We use bacteriophage φ6, a member of the Cystoviridae family, as a model system to study the assembly of a complicated multi-shelled virus. The inner T=1 shell, composed of protein P1, forms a dodecahedral polymerase complex (PC) harbouring the three viral dsRNA segments (S, M, and L), the viral polymerase P2, the hexameric packaging protein P4, and the assembly cofactor P7. The expanded PC is covered by a layer of P8, forming the outer T=13 shell. Here we present the structure of φ6 NC to near-atomic resolution using electron cryomicroscopy and single particle analysis.

The six-fold symmetry of the P4 hexamer and five-fold symmetry of the icosahedral vertex beneath creates a symmetry mismatch, so that the structure of P4 cannot be resolved using conventional icosahedral reconstruction. To address this we applied the localized reconstruction method17 to P4 hexamers. Local areas corresponding to P4 hexamers were extracted from the NC images and reconstructed as single particles with six-fold symmetry (‘P4 hexamer reconstruction') or without any symmetry (‘NC vertex reconstruction'). This allowed a low-resolution structure of the P4 hexamer to be determined in situ. Our localized reconstruction of P4 hexamers that correctly dealt with the symmetry mismatch revealed elongated densities extending from 3 of the 6 P4 C-terminal parts. We hypothesised that these may correspond to the C-terminal parts that are disordered in the crystal structure. The sixth, unbound C-terminal region of P4 was not resolved in any of the reconstructions, and is likely to be either disordered or unresolved in our maps due to limited resolution of the localized reconstructions. Binding of up to five of the six flexible C-terminal tails of P4 provides an elegant solution to the symmetry mismatch.

>MPIVVTQAHIDRVGIAADLLDASPVSLQVLGRPTAINTVVIKTYIAAVMELASKQGGSLAGVDIRPSVLLKDTAIFTKPKAKSADVESDVDVLDTGIYSVPGLARKPVTHRWPSEGIYSGVTALMGATGSGKSITLNEKLRPDVLIRWGEVAEAYDELDTAVHISTLDEMLIVCIGLGALGFNVAVDSVRPLLFRLKGAASAGGIVAVFYSLLTDISNLFTQYDCSVVMVVNPMVDAEKIEYVFGQVMASTVGAILCADGNVSRTMFRTNKGRIFNGAAPLAADTHMPSMDRPTSMKALDHTSIASVAP[6x]> GATAEKQKHDGRVKIGHYILGDTLGVGTFGKVKVGKHELTGHKVAVKILNRQKIRSLDVVGKIRREIQNLKLFRHPHIIKLYQVISTPSDIFMV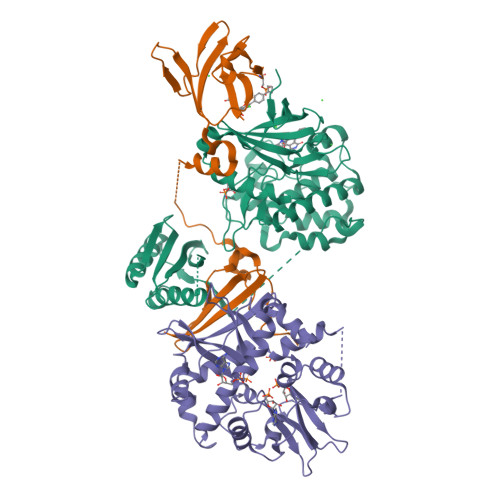MEYVSGGELFDYICKNGRLDEKESRRLFQQILSGVDYCHRHMVVHRDLKPENVLLDAHMNAKIADFGLSNMMSDGEFLRTSCGSPNYAAPEVISGRLYAGPEVDIWSSGVILYALLCGTLPFDDDHVPTLFKKICDGIFYTPQYLNPSVISLLKHMLQVDPMKRATIKDIREHEWFKQDLPKYLFPEDPSYSSTMIDDEALKEVCEKFECSEEEVLSCLYNRNHQDPLAVAYHLIIDNRRIMNEAKDFYLATSPPDSFLDDHHLTRPHPERVPFLVAETPRARHTLDELNPQKSKHQGVRKAKWHLGIRSQSRPNDIMAEVCRAIKQLDYEWKVVNPYYLRVRRKNPVTSTFSKMSLQLYQVDSRTYLLDFRSIDDEASGGPGGSAPRPGSHTIEFFEMCANLIKILAQ;> MEVNEKAPAQARPTVFRWTGGGKEVYLSGSFNNWSKLPLTRSQNNFVAILDLPEGEHQYKFFVDGQWTHDPSEPIVTSQLGTVNNIIQVKKTDFEVFDALMVDSQKCSDVSELSSSPPGPYHQEPYISKPEERFKAPPILPPHLLQVILNKDTGISCDPALLPEPNHVMLNHLYALSIKDGVMVLSATHRYKKKYVTTLLYKPI;> MESVAAESAPAPENEHSQETPESNSSVYTTFMKSHRCYDLIPTSSKLVVFDTSLQVKKAFFALVTNGVRAAPLWDSKKQSFVGMLTITDFINILHRYYKSALVQIYELEEHKIETWREVYLQDSFKPLVCISPNASLFDAVSSLIRNKIHRLPVIDPESGNTLYILTHKRILKFLKLFITEFPKPEFMSKSLEELQIGTYANIAMVRTTTPVYVALGIFVQHRVSALPVVDEKGRVVDIYSKFDVINLAAEKTYNNLDVSVTKALQHRSHYFEGVLKCYLHETLEAIINRLVEAEVHRLVVVDEHDVVKGIVSLSDILQALVLTGGEKKP>[2x]MKCLVVGHVVRDIVKKGNKVLERLGGGAYYSALALSRFCDV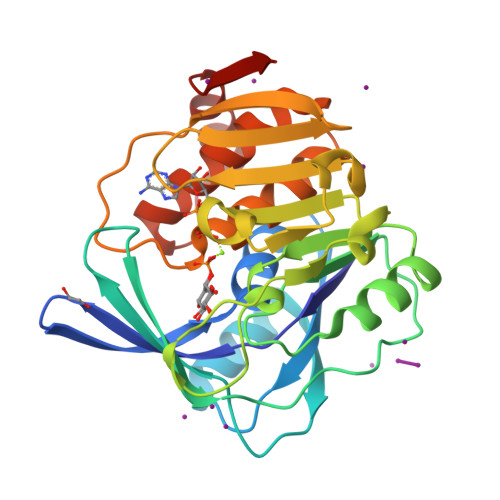EILTSFSNLPEEWIKELESMAKLQVVPSETTTTYELTYLDGNRRRLKLLERASPIEELPDGEYDVLLMNPVAREVPPALVTSALKKFPFVAVDIQGFIRSSSPGEIQYQPIDGSFLKGVKILHADLGEYQYLQGFSPEFVDVLLLSNGPEPGKAFLHGREYTFEPVHVGVDESTGAGDVFLGAFTGFYSQCPFVQALKRAAAFTALFLKNRSVDFSMDDVNELAMKVEVKRV> SGMGCIT

Although other intermediate filament proteins have been demonstrated to form amyloids, KRT8 specifically has not previously been characterized as an amyloid-forming protein. This protein, like other alpha-keratin proteins, contains a central coiled-coil domain that is flanked by an amino-terminal head domain and a carboxy-terminal tail domain, which are both low complexity in sequence composition. KRT8 is known to aggregate pathologically, primarily in the form of MDBs in liver disease. Atomic structures of KRT8 LARKS reveal that pathogenic mutations convert the non-pleated wild-type protein into a pleated conformation, shedding light on the molecular mechanisms underlying aggregation-promoting mutations in low-complexity proteins.

For experimental validation, we selected three of these KRT8 mutants (G62C, Y54H, and G55A), all of which are found in people with cryptogenic liver disease, as well as three FUS mutants (G191S, G225V, and G230C). To assess the structural impacts of the disease-associated mutations, we determined the atomic structures of several LARKS from KRT8 for both the wild-type and mutant sequences. Segment crystal structures of KRT858–64 (wild type: SGMGGIT; G62C: SGMGCIT) for the wild-type protein and KRT8-G62C were determined. The G62C mutant fibril is a parallel beta-sheet, whose steric-zipper interface is driven by hydrophobic interactions between Met60, Cys62, and Ile63. c, The KRT852–58-G55A mutant structure GGYAGAS was also determined, revealing an anti-parallel beta-sheet with a steric-zipper interface formed by Tyr54, Ala55, and Ala57. d, Alignment of the wild-type and mutant KRT858–64 segments shows a transition in backbone conformation from a highly extended to a pleated beta-sheet at the site of the mutation (circled). Alignment of the beta-strands from both structures highlights that the G62C mutation results in the non-pleated Gly62 converting to a pleated conformation as Cys62 (shown in inset). e, Comparison of the KRT852-58-G55A GGYAGAS segment with a structure from hnRNPA1 whose sequences closely match the corresponding KRT8 wild-type (hnRNPA1: GGGYGGS versus KRT8: GGYGGAS) shows a similar trend in transitioning from an extended beta-sheet in the wild type to a pleated conformation in the mutant. From these fibril structures, we observe that both the G62C and G55A mutations in KRT8 convert a non-pleated beta-sheet into a pleated one, transitioning a LARKS-like conformation into a steric zipper. Suggesting an effect of alcohol on KRT8 aggregation, two of three of our crystal structures of KRT8 segments showed the peptides in complex with either ethanol or isopropanol, each with distinct binding sites.>NGSEWSYTNILTGPETWHEHYKNMCSGYYQSPIDLKTDISTLDLKLKTVIIYRNTSSTETTTIQNNGHSAEVKFPRNTWFISFDGILDYKYEIIQMHFHWGNTDDRGSEHTIDGFRFPLEGHIVSFRRQMYSSPSEAIGRPGGLAVLGIMHQIVESIKYEQTAFKAYNNFSGVLNSQFVPPNNSTIDDINLALLLSLLNPSRYFRYLGSLTTPPCTENVLWTVFIDPVLITREQINLFRNLPYGSNEKQTRMGDNFRPIQLLNPIDTLAS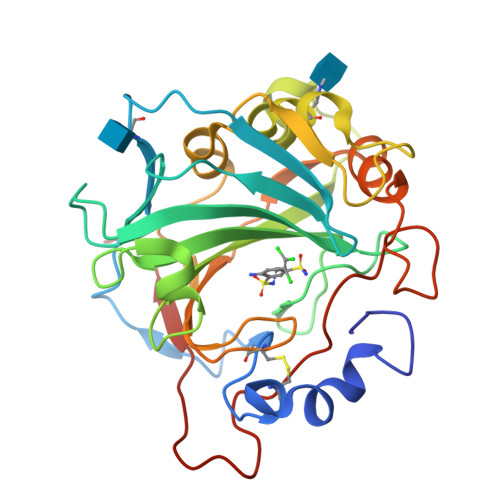RTLYRATARG[2x]>MRGSHHHHHHGSMSYYNLEKDDTVYYKLDTIKCDIPINEELQARINKHVNQLRITYSTLEEFVDNFVYELKKGLEAHRRHPNLWIPHECSFKMLDSCIADIPTGQEKGTYYAIDFGGTNFRAVRASLDGNGKIKRDQETYSLKFTGTFSHEKGLLDKHATASQLFDHFAERIKYIMGEFKDLDNPEGKNVGFTFSFPCTSPSINCSILIDWTKGFETGRATNDPVEGRDVCKLMNDAFVRSEVPAKVCCVVNDAVGTLMSCAYQKGKTTPPCYIGIIL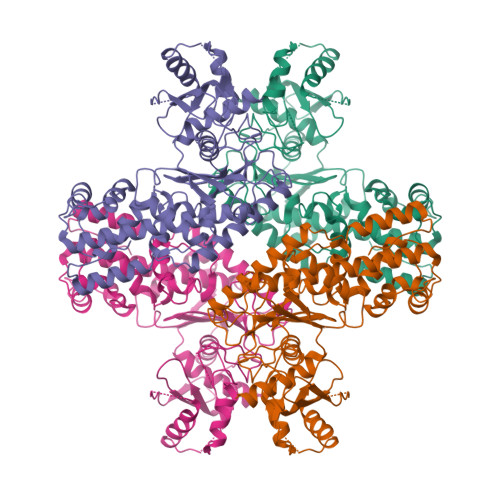GTGSNGCYYEPEWKKYKYSGKIINIELGNFDKDLPLSPIDLVMDWHSANRSRQLFEKMISGAYLGEIVRRFMVNVLQSASSEKMWKSDSFNSELGSVVLNDTSPNFEESRKVAKDAWDMDFTDEQIYALRKICESVYNRSAALAAAAIAAIAKRIKIIEHSKFSCGVDGSLFVKNAWYCKRLQEHLKVILADKAENLIIIPADDGSGKGAAITAAVVSQSSSIKQLP[4x]> HMASMKKKGSVVIVGRINLSGDTAYAQQTRGEEGCQETSQTGRDKNQVEGEVQIVSTATQTFLATSINGVLWTVYHGAGTRTIASPKGPVTQMYTNVDKDLVGWQAPQGSRSLTPCTCGSSDLYLVTRHADVIPVRRRGDSTGSLLSPRPLSYLKGSSGGPLLCPAGHAVGIF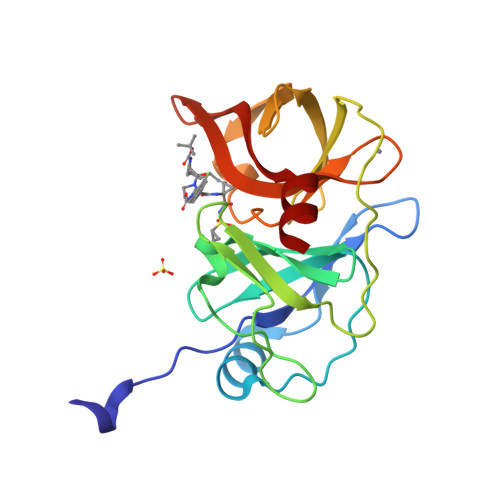RAAVSTRGVAKAVQFIPVESLETTM> SPTVEECGYSDRVRSITLGNSTITTQECANVVVGYGVWPDYLKDSEATAEDQPTQPDVATCRFYTLDSVQWQKTSPGWWWKLPDALSNLGLFGQNMQYHYLGRTGYTIHV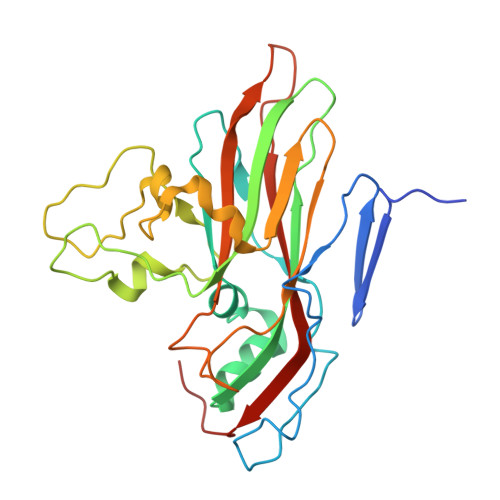QCNASKFHQGCLLVVCVPEAEMGCATLDNTPSSAELLGGDAAKEFAGEPIASGSNKLVQRVVYNAGMGIGVGNLTIFPHQWINLRTNNSATIVMPYTNSVPMDNMFRHNNITLMVIPFVPLDYCPGSTTYVPITVTIAPMCAEYNGLRLASHQ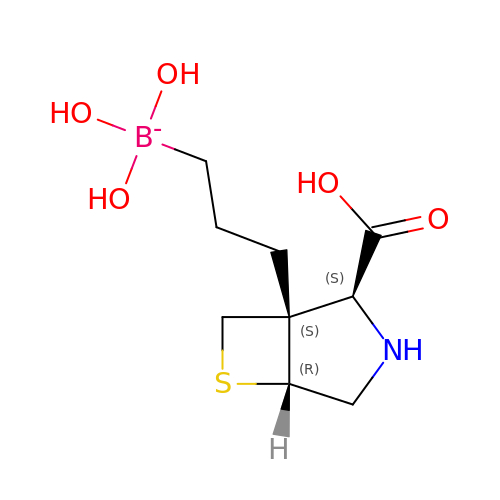3-[(1~{S},2~{S},5~{R})-2-carboxy-6-thia-3-azabicyclo[3.2.0]heptan-1-yl]propyl-$l^{3}-oxidanyl-bis(oxidanyl)boranuide | C9 H17 B N O5 S | UPRXFJNZWUYSLX-OOZYFLPDSA-N methyl 4-chloranyl-2-(phenylsulfonyl)-5-sulfamoyl-benzoate | C14 H12 Cl 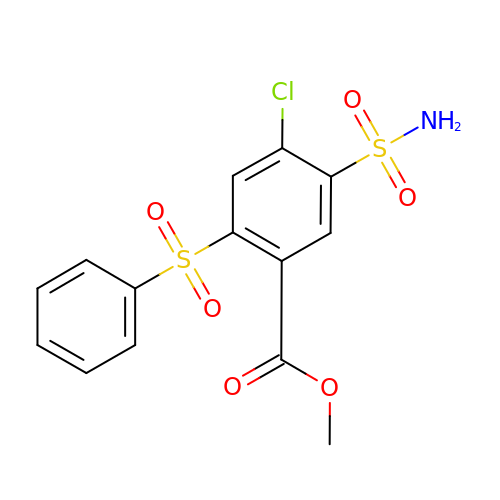N O6 S2 | IGXGTYUIRLTUTM-UHFFFAOYSA-N>[2x]MEFTTGLMSLDTALNEMLSRVTPL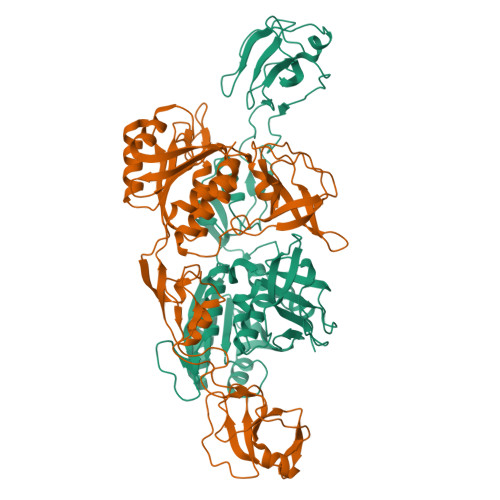TAQETLPLVQCFGRILASDVVSPLDVPGFDNSAMDGYAVRLADIASGQPLPVAGKSFAGQPYHGEWPAGTCIRIMTGAPVPEGCEAVVMQEQTEQMDNGVRFTAEVRSGQNIRRRGEDISAGAVVFPAGTRLTTAELPVIASLGIAEVPVIRKVRVALFSTGDELQLPGQPLGDGQIYDTNRLAVHLMLEQLGCEVINLGIIRDDPHALRAAFIEADSQADVVISSGGVSVGEADYTKTILEELGEIAFWKLAIKPGKPFAFGKLSNSWFCGLPGNPVSATLTFYQLVQPLLAKLSGNTASGLPARQRVRTASRLKKTPGRLDFQRGVLQRNADGELEVTTTGHQGWHIFSSFSLGNCFIVLERDRGNVEVGEWVEVEPFNALFGGL> GHMNSFVGLRVVAKWSSNGYFYSGKITRDVGAGKYKLLFDDGYECDVLGKDILLCDPIPLDTEVTALSEDEYFSAGVVKGHRKESGELYYSIEKEGQRKWYKRMAVILSLEQGNRLREQYGLG;> KRH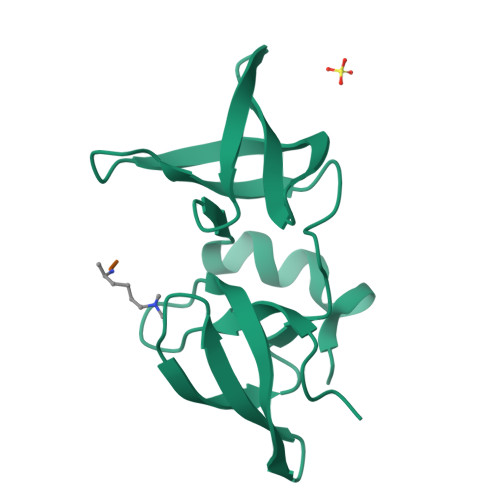RKVLRDN>[2x]MFKDGSLIPYLTAGDPNKQSTLNFLLALDEYAGAIELGIPFSDPIADGKTIQE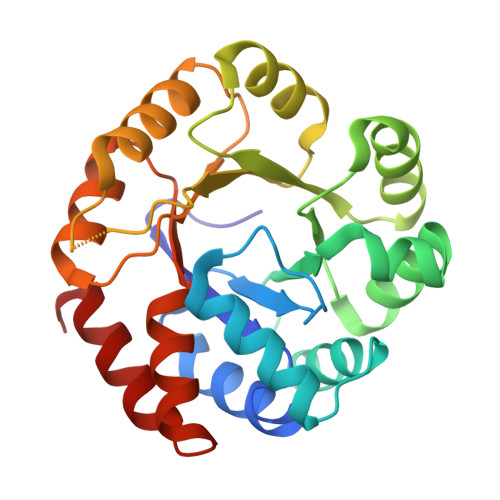SHYRALKNGFKLREAFWIVKEFRRHSSTPIVLMTYYNPIYRAGVRNFLAEAKASGVDGILVVDLPVFHAKEFTEIAREEGIKTVFLAAPNTPDERLKVIDDMTTGFVYLVSLYGTTGAREEIPKTAYDLLRRAKRICRNKVAVGFGVSKREHVVSLLKEGANGVVVGSALVKIIGEKGREATEFLKKKVEELLGI> NQAVREFAKEIDASCIKIEKVIGVGEFGEVCSGRLKVPGKREICVAIKTLKAGYTDKQRRDFLSEASIMGQFDHPNIIHLEGVVTKCKPVMIITEYMENGSLDAFLRKNDGRFTVIQLVGMLRGIGSGMKYLSDMSYVHRDLAARNILVNSNLVCKVSD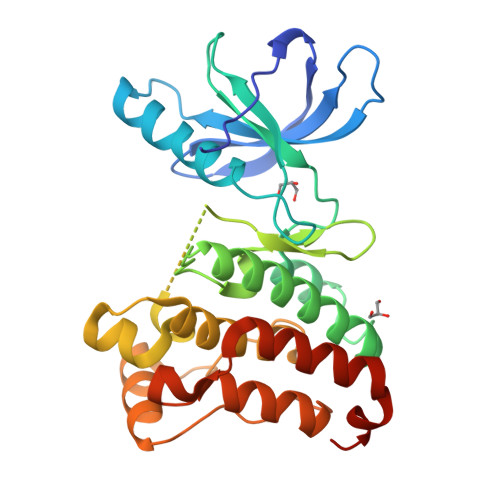FGMSRVLEDDPEAAYTTRGGKIPIRWTAPEAIAYRKFTSASDVWSYGIVMWEVMSYGERPYWDMSNQDVIKAIEEGYRLPPPMDCPIALHQLMLDCWQKERSDRPKFGQIVNMLDKLIRNPNSLKRTGSESS> PNFSGNWKIIRSENFEELLKVLGVNVMLRKIAVAAASKYAVEIKQEGDTFYIKVSTTVYTTEINFKVGEEFEEQTVDGRPCKSLVKWESENKMVCEQKLLKGEGPKTSWTKELTNDGELIYTMTADDVVCTQVF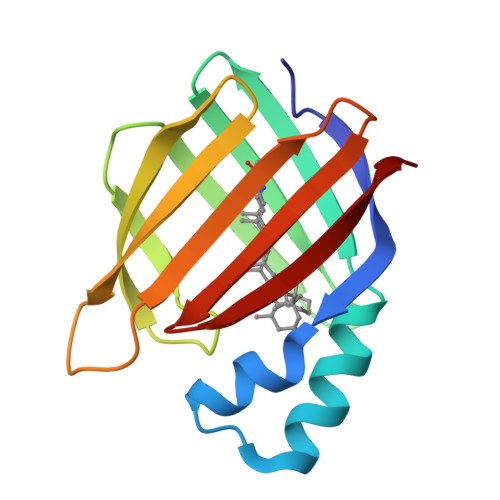VRE> MCCLYTSDVFFWSSLVVSPLPRIVRCVSAPQIRSIPCGSGDFSVMKRSLIARWQSGVHTPHGVVYRGAKMKNWPEQRIPENFKFTEEQRFRTKAIPRDVGTIPRNFVLGVL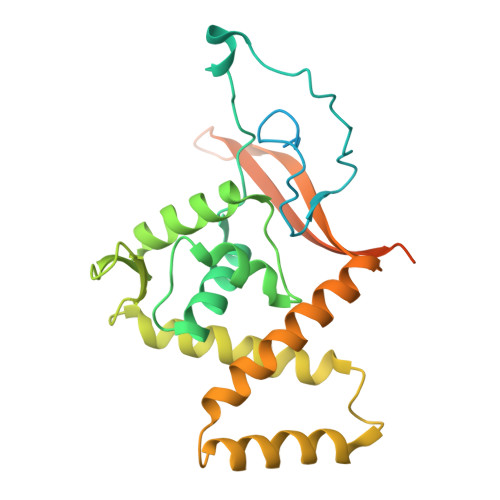YRHQPCEVGGLWEHCTNDPEIVLDSKRHLREVLKQAREEGFVTFERDAISNEWLCFLTRERYEEVQRIVTAKSEAVDSSSSSSSSSSSSSSSSSSSSSSSSSSSSSSHARRLEEEVANTTRYLRRFQQREIDYLPYTDLNGKVNFMWWYETRDVQQRADEVLTDSSSSKALAGEEEHKAGSQLEATTASTS> GSHMDRYDIAIIGSGPAGLSAAINAVIRNKKVILFGSDNLSNKLLKAPKINNYLGIYDVSGKELKEK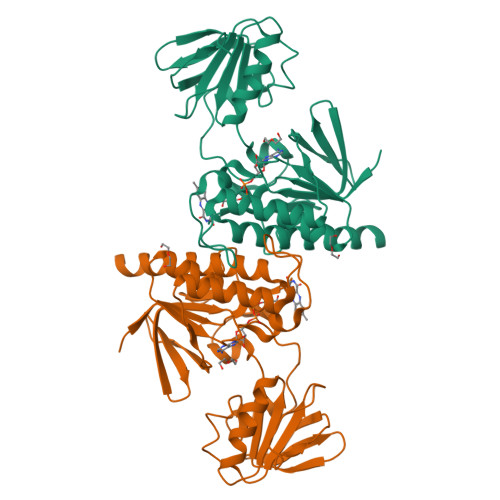FLEHLKYMNIEIKNEKVNSVYSMGDYFALSLNQKMYEATSIIIASGVEFSKPLNGEDELLGKGVGYCATCDAPLYKGKTVAIVGYTKEAEEEANYVSELAGKLYYIPMYKDKVSLKEVIEVVEDKPISILGKDKVSGLQMSKGEINTDAVFIIKDSVSPGKLVPGLLMNGEHIAVDIDMKTNIEGCFAAGDCAGRPYQYIKSAGQGQIAALSAVSYIDKIKLNKKII> MTKENICIVFGGKSAEHEVSILTAQN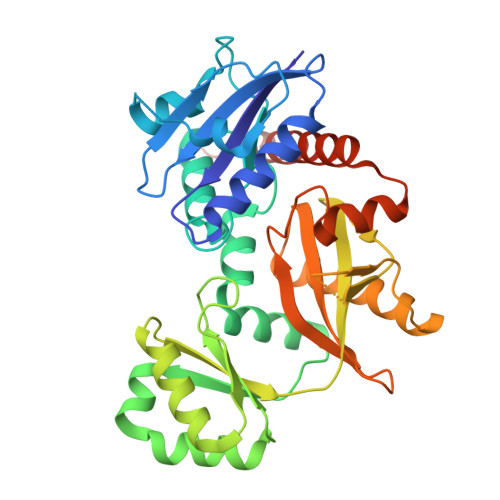VLNAIDKDKYHVDIIYITNDGDWRKQNNITAEIKSTDELHLENGEALEISQLLKESSSGQPYDAVFPLLHGPNGEDGTIQGLFEVLDVPYVGNGVLSAASSMDKLVMKQLFEHRGLPQLPYISFLRSEYEKYEHNILKLVNDKLNYPVFVKPANLGSSVGISKCNNEAELKEGIKEAFQFDRKLVIEQGVNAREIEVAVLGNDYPEATWPGEVVKDVAFYDYKSKYKDGKVQLQIPADLDEDVQLTLRNMALEAFKATDCSGLVRADFFVTEDNQIYINETNAMPGFTAFSMYPKLWENMGLSYPELITKLIELAKERHQDKQKNKYKIDRSHHHHHH> CTTTACCCTACTGGTAAATCCGCGACCTGCTC;> AAACGAGATTGAGTAAACATCGACGGATAGCTATACCGGGGGTTTCTG;> GAACCGCCCCCCCTGCCTCATTTGCCGCCAGCCGGCCAGAGGGTTACC;> GTATAAACGTACCAGGTATAGCCCGGAATAGGGTCACCAGGAATCCCCTGCGGGAT;> CTATTTCGGAACCTATGAGAAGGAGGAGGTTTGGCTGAGATTTTT;> TGATGATAAATGCCGGGAAAGGGGCTCTTCGCTATTACGCCAAGAGAA;> ATGGCTTTTAACGGGGTCAGTGCCATGACCAT;> TAAAGCCAATTCACAACCACCCTCAGAGCCGC;> CACGACGTCGTTTTAAAACGAGGCGCAGACGG;> CGGAAACATCCCGGAATTTGTGAGGGATCCCCATGCGGCGAAAGAAAC;> TGATAGACGGTTTTTCGCCCTTTGACGTTGGAGTCCACGTTCTTTAATAGTGGACTCTTGTTCCAAACTGGAACAACACTCAACCCTATCTCGGGCTATTCTTTTGATTTATAAGGGATTTTGCCGATTTCGGAACCACCATCAAACAGGATTTTCGCCTGCTGGGGCAAACCAGCGTGGACCGCTTGCTGCAACTCTCTCAGGGCCAGGCGGTGAAGGGCAATCAGCTGTTGCCCGTCTCACTGGTGAAAAGAAAAACCACCCTGGCGCCCAATACGCAAACCGCCTCTCCCCGCGCGTTGGCCGATTCATTAATGCAGCTGGCACGACAGGTTTCCCGACTGGAAAGCGGGCAGTGAGCGCAACGCAATTAATGTGAGTTAGCTCACTCATTAGGCACCCCAGGCTTTACACTTTATGCTTCCGGCTCGTATGTTGTGTGGAATTGTGAGCGGATAACAATTTCACACAGGAAACAGCTATGACCATGATTACGAATTCGAGCTCGGTACCCGGGGATCCTCAACTGTGAGGAGGCTCACGGACGCGAAGAACAGGCACGCGTGCTGGCAGAAACCCCCGGTATGACCGTGAAAACGGCCCGCCGCATTCTGGCCGCAGCACCACAGAGTGCACAGGCGCGCAGTGACACTGCGCTGGATCGTCTGATGCAGGGGGCACCGGCACCGCTGGCTGCAGGTAACCCGGCATCTGATGCCGTTAACGATTTGCTGAACACACCAGTGTAAGGGATGTTTATGACGAGCAAAGAAACCTTTACCCATTACCAGCCGCAGGGCAACAGTGACCCGGCTCATACCGCAACCGCGCCCGGCGGATTGAGTGCGAAAGCGCCTGCAATGACCCCGCTGATGCTGGACACCTCCAGCCGTAAGCTGGTTGCGTGGGATGGCACCACCGACGGTGCTGCCGTTGGCATTCTTGCGGTTGCTGCTGACCAGACCAGCACCACGCTGACGTTCTACAAGTCCGGCACGTTCCGTTATGAGGATGTGCTCTGGCCGGAGGCTGCCAGCGACGAGACGAAAAAACGGACCGCGTTTGCCGGAACGGCAATCAGCATCGTTTAACTTTACCCTTCATCACTAAAGGCCGCCTGTGCGGCTTTTTTTACGGGATTTTTTTATGTCGATGTACACAACCGCCCAACTGCTGGCGGCAAATGAGCAGAAATTTAAGTTTGATCCGCTGTTTCTGCGTCTCTTTTTCCGTGAGAGCTATCCCTTCACCACGGAGAAAGTCTATCTCTCACAAATTCCGGGACTGGTAAACATGGCGCTGTACGTTTCGCCGATTGTTTCCGGTGAGGTTATCCGTTCCCGTGGCGGCTCCACCTCTGAAAGCTTGGCACTGGCCGTCGTTTTACAACGTCGTGACTGGGAAAACCCTGGCGTTACCCAACTTAATCGCCTTGCAGCACATCCCCCTTTCGCCAGCTGGCGTAATAGCGAAGAGGCCCGCACCGATCGCCCTTCCCAACAGTTGCGCAGCCTGAATGGCGAATGGCGCTTTGCCTGGTTTCCGGCACCAGAAGCGGTGCCGGAAAGCTGGCTGGAGTGCGATCTTCCTGAGGCCGATACTGTCGTCGTCCCCTCAAACTGGCAGATGCACGGTTACGATGCGCCCATCTACACCAACGTGACCTATCCCATTACGGTCAATCCGCCGTTTGTTCCCACGGAGAATCCGACGGGTTGTTACTCGCTCACATTTAATGTTGATGAAAGCTGGCTACAGGAAGGCCAGACGCGAATTATTTTTGATGGCGTTCCTATTGGTTAAAAAATGAGCTGATTTAACAAAAATTTAATGCGAATTTTAACAAAATATTAACGTTTACAATTTAAATATTTGCTTATACAATCTTCCTGTTTTTGGGGCTTTTCTGATTATCAACCGGGGTACATATGATTGACATGCTAGTTTTACGATTACCGTTCATCGATTCTCTTGTTTGCTCCAGACTCTCAGGCAATGACCTGATAGCCTTTGTAGATCTCTCAAAAATAGCTACCCTCTCCGGCATTAATTTATCAGCTAGAACGGTTGAATATCATATTGATGGTGATTTGACTGTCTCCGGCCTTTCTCACCCTTTTGAATCTTTACCTACACATTACTCAGGCATTGCATTTAAAATATATGAGGGTTCTAAAAATTTTTATCCTTGCGTTGAAATAAAGGCTTCTCCCGCAAAAGTATTACAGGGTCATAATGTTTTTGGTACAACCGATTTAGCTTTATGCTCTGAGGCTTTATTGCTTAATTTTGCTAATTCTTTGCCTTGCCTGTATGATTTATTGGATGTTAATGCTACTACTATTAGTAGAATTGATGCCACCTTTTCAGCTCGCGCCCCAAATGAAAATATAGCTAAACAGGTTATTGACCATTTGCGAAATGTATCTAATGGTCAAACTAAATCTACTCGTTCGCAGAATTGGGAATCAACTGTTATATGGAATGAAACTTCCAGACACCGTACTTTAGTTGCATATTTAAAACATGTTGAGCTACAGCATTATATTCAGCAATTAAGCTCTAAGCCATCCGCAAAAATGACCTCTTATCAAAAGGAGCAATTAAAGGTACTCTCTAATCCTGACCTGTTGGAGTTTGCTTCCGGTCTGGTTCGCTTTGAAGCTCGAATTAAAACGCGATATTTGAAGTCTTTCGGGCTTCCTCTTAATCTTTTTGATGCAATCCGCTTTGCTTCTGACTATAATAGTCAGGGTAAAGACCTGATTTTTGATTTATGGTCATTCTCGTTTTCTGAACTGTTTAAAGCATTTGAGGGGGATTCAATGAATATTTATGACGATTCCGCAGTATTGGACGCTATCCAGTCTAAACATTTTACTATTACCCCCTCTGGCAAAACTTCTTTTGCAAAAGCCTCTCGCTATTTTGGTTTTTATCGTCGTCTGGTAAACGAGGGTTATGATAGTGTTGCTCTTACTATGCCTCGTAATTCCTTTTGGCGTTATGTATCTGCATTAGTTGAATGTGGTATTCCTAAATCTCAACTGATGAATCTTTCTACCTGTAATAATGTTGTTCCGTTAGTTCGTTTTATTAACGTAGATTTTTCTTCCCAACGTCCTGACTGGTATAATGAGCCAGTTCTTAAAATCGCATAAGGTAATTCACAATGATTAAAGTTGAAATTAAACCATCTCAAGCCCAATTTACTACTCGTTCTGGTGTTTCTCGTCAGGGCAAGCCTTATTCACTGAATGAGCAGCTTTGTTACGTTGATTTGGGTAATGAATATCCGGTTCTTGTCAAGATTACTCTTGATGAAGGTCAGCCAGCCTATGCGCCTGGTCTGTACACCGTTCATCTGTCCTCTTTCAAAGTTGGTCAGTTCGGTTCCCTTATGATTGACCGTCTGCGCCTCGTTCCGGCTAAGTAACATGGAGCAGGTCGCGGATTTCGACACAATTTATCAGGCGATGATACAAATCTCCGTTGTACTTTGTTTCGCGCTTGGTATAATCGCTGGGGGTCAAAGATGAGTGTTTTAGTGTATTCTTTTGCCTCTTTCGTTTTAGGTTGGTGCCTTCGTAGTGGCATTACGTATTTTACCCGTTTAATGGAAACTTCCTCATGAAAAAGTCTTTAGTCCTCAAAGCCTCTGTAGCCGTTGCTACCCTCGTTCCGATGCTGTCTTTCGCTGCTGAGGGTGACGATCCCGCAAAAGCGGCCTTTAACTCCCTGCAAGCCTCAGCGACCGAATATATCGGTTATGCGTGGGCGATGGTTGTTGTCATTGTCGGCGCAACTATCGGTATCAAGCTGTTTAAGAAATTCACCTCGAAAGCAAGCTGATAAACCGATACAATTAAAGGCTCCTTTTGGAGCCTTTTTTTTGGAGATTTTCAACGTGAAAAAATTATTATTCGCAATTCCTTTAGTTGTTCCTTTCTATTCTCACTCCGCTGAAACTGTTGAAAGTTGTTTAGCAAAATCCCATACAGAAAATTCATTTACTAACGTCTGGAAAGACGACAAAACTTTAGATCGTTACGCTAACTATGAGGGCTGTCTGTGGAATGCTACAGGCGTTGTAGTTTGTACTGGTGACGAAACTCAGTGTTACGGTACATGGGTTCCTATTGGGCTTGCTATCCCTGAAAATGAGGGTGGTGGCTCTGAGGGTGGCGGTTCTGAGGGTGGCGGTTCTGAGGGTGGCGGTACTAAACCTCCTGAGTACGGTGATACACCTATTCCGGGCTATACTTATATCAACCCTCTCGACGGCACTTATCCGCCTGGTACTGAGCAAAACCCCGCTAATCCTAATCCTTCTCTTGAGGAGTCTCAGCCTCTTAATACTTTCATGTTTCAGAATAATAGGTTCCGAAATAGGCAGGGGGCATTAACTGTTTATACGGGCACTGTTACTCAAGGCACTGACCCCGTTAAAACTTATTACCAGTACACTCCTGTATCATCAAAAGCCATGTATGACGCTTACTGGAACGGTAAATTCAGAGACTGCGCTTTCCATTCTGGCTTTAATGAGGATTTATTTGTTTGTGAATATCAAGGCCAATCGTCTGACCTGCCTCAACCTCCTGTCAATGCTGGCGGCGGCTCTGGTGGTGGTTCTGGTGGCGGCTCTGAGGGTGGTGGCTCTGAGGGTGGCGGTTCTGAGGGTGGCGGCTCTGAGGGAGGCGGTTCCGGTGGTGGCTCTGGTTCCGGTGATTTTGATTATGAAAAGATGGCAAACGCTAATAAGGGGGCTATGACCGAAAATGCCGATGAAAACGCGCTACAGTCTGACGCTAAAGGCAAACTTGATTCTGTCGCTACTGATTACGGTGCTGCTATCGATGGTTTCATTGGTGACGTTTCCGGCCTTGCTAATGGTAATGGTGCTACTGGTGATTTTGCTGGCTCTAATTCCCAAATGGCTCAAGTCGGTGACGGTGATAATTCACCTTTAATGAATAATTTCCGTCAATATTTACCTTCCCTCCCTCAATCGGTTGAATGTCGCCCTTTTGTCTTTGGCGCTGGTAAACCATATGAATTTTCTATTGATTGTGACAAAATAAACTTATTCCGTGGTGTCTTTGCGTTTCTTTTATATGTTGCCACCTTTATGTATGTATTTTCTACGTTTGCTAACATACTGCGTAATAAGGAGTCTTAATCATGCCAGTTCTTTTGGGTATTCCGTTATTATTGCGTTTCCTCGGTTTCCTTCTGGTAACTTTGTTCGGCTATCTGCTTACTTTTCTTAAAAAGGGCTTCGGTAAGATAGCTATTGCTATTTCATTGTTTCTTGCTCTTATTATTGGGCTTAACTCAATTCTTGTGGGTTATCTCTCTGATATTAGCGCTCAATTACCCTCTGACTTTGTTCAGGGTGTTCAGTTAATTCTCCCGTCTAATGCGCTTCCCTGTTTTTATGTTATTCTCTCTGTAAAGGCTGCTATTTTCATTTTTGACGTTAAACAAAAAATCGTTTCTTATTTGGATTGGGATAAATAATATGGCTGTTTATTTTGTAACTGGCAAATTAGGCTCTGGAAAGACGCTCGTTAGCGTTGGTAAGATTCAGGATAAAATTGTAGCTGGGTGCAAAATAGCAACTAATCTTGATTTAAGGCTTCAAAACCTCCCGCAAGTCGGGAGGTTCGCTAAAACGCCTCGCGTTCTTAGAATACCGGATAAGCCTTCTATATCTGATTTGCTTGCTATTGGGCGCGGTAATGATTCCTACGATGAAAATAAAAACGGCTTGCTTGTTCTCGATGAGTGCGGTACTTGGTTTAATACCCGTTCTTGGAATGATAAGGAAAGACAGCCGATTATTGATTGGTTTCTACATGCTCGTAAATTAGGATGGGATATTATTTTTCTTGTTCAGGACTTATCTATTGTTGATAAACAGGCGCGTTCTGCATTAGCTGAACATGTTGTTTATTGTCGTCGTCTGGACAGAATTACTTTACCTTTTGTCGGTACTTTATATTCTCTTATTACTGGCTCGAAAATGCCTCTGCCTAAATTACATGTTGGCGTTGTTAAATATGGCGATTCTCAATTAAGCCCTACTGTTGAGCGTTGGCTTTATACTGGTAAGAATTTGTATAACGCATATGATACTAAACAGGCTTTTTCTAGTAATTATGATTCCGGTGTTTATTCTTATTTAACGCCTTATTTATCACACGGTCGGTATTTCAAACCATTAAATTTAGGTCAGAAGATGAAATTAACTAAAATATATTTGAAAAAGTTTTCTCGCGTTCTTTGTCTTGCGATTGGATTTGCATCAGCATTTACATATAGTTATATAACCCAACCTAAGCCGGAGGTTAAAAAGGTAGTCTCTCAGACCTATGATTTTGATAAATTCACTATTGACTCTTCTCAGCGTCTTAATCTAAGCTATCGCTATGTTTTCAAGGATTCTAAGGGAAAATTAATTAATAGCGACGATTTACAGAAGCAAGGTTATTCACTCACATATATTGATTTATGTACTGTTTCCATTAAAAAAGGTAATTCAAATGAAATTGTTAAATGTAATTAATTTTGTTTTCTTGATGTTTGTTTCATCATCTTCTTTTGCTCAGGTAATTGAAATGAATAATTCGCCTCTGCGCGATTTTGTAACTTGGTATTCAAAGCAATCAGGCGAATCCGTTATTGTTTCTCCCGATGTAAAAGGTACTGTTACTGTATATTCATCTGACGTTAAACCTGAAAATCTACGCAATTTCTTTATTTCTGTTTTACGTGCAAATAATTTTGATATGGTAGGTTCTAACCCTTCCATTATTCAGAAGTATAATCCAAACAATCAGGATTATATTGATGAATTGCCATCATCTGATAATCAGGAATATGATGATAATTCCGCTCCTTCTGGTGGTTTCTTTGTTCCGCAAAATGATAATGTTACTCAAACTTTTAAAATTAATAACGTTCGGGCAAAGGATTTAATACGAGTTGTCGAATTGTTTGTAAAGTCTAATACTTCTAAATCCTCAAATGTATTATCTATTGACGGCTCTAATCTATTAGTTGTTAGTGCTCCTAAAGATATTTTAGATAACCTTCCTCAATTCCTTTCAACTGTTGATTTGCCAACTGACCAGATATTGATTGAGGGTTTGATATTTGAGGTTCAGCAAGGTGATGCTTTAGATTTTTCATTTGCTGCTGGCTCTCAGCGTGGCACTGTTGCAGGCGGTGTTAATACTGACCGCCTCACCTCTGTTTTATCTTCTGCTGGTGGTTCGTTCGGTATTTTTAATGGCGATGTTTTAGGGCTATCAGTTCGCGCATTAAAGACTAATAGCCATTCAAAAATATTGTCTGTGCCACGTATTCTTACGCTTTCAGGTCAGAAGGGTTCTATCTCTGTTGGCCAGAATGTCCCTTTTATTACTGGTCGTGTGACTGGTGAATCTGCCAATGTAAATAATCCATTTCAGACGATTGAGCGTCAAAATGTAGGTATTTCCATGAGCGTTTTTCCTGTTGCAATGGCTGGCGGTAATATTGTTCTGGATATTACCAGCAAGGCCGATAGTTTGAGTTCTTCTACTCAGGCAAGTGATGTTATTACTAATCAAAGAAGTATTGCTACAACGGTTAATTTGCGTGATGGACAGACTCTTTTACTCGGTGGCCTCACTGATTATAAAAACACTTCTCAGGATTCTGGCGTACCGTTCCTGTCTAAAATCCCTTTAATCGGCCTCCTGTTTAGCTCCCGCTCTGATTCTAACGAGGAAAGCACGTTATACGTGCTCGTCAAAGCAACCATAGTACGCGCCCTGTAGCGGCGCATTAAGCGCGGCGGGTGTGGTGGTTACGCGCAGCGTGACCGCTACACTTGCCAGCGCCCTAGCGCCCGCTCCTTTCGCTTTCTTCCCTTCCTTTCTCGCCACGTTCGCCGGCTTTCCCCGTCAAGCTCTAAATCGGGGGCTCCCTTTAGGGTTCCGATTTAGTGCTTTACGGCACCTCGACCCCAAAAAACTTGATTTGGGTGATGGTTCACGTAGTGGGCCATCGCCC;> TTCGCCATTCAGGCTGCCAGCTTTTTTTT;> TCGATGAACGGTAATCAAGCGCCAGGCGATCGCAGTTTGATTCTAGCT;> TTTTTGGAGCAAACTACAAAGCATTGCCTGCTATTTTAAAAGGGTGAGAAAGG;> TTTTCCGGCACCTCGGCCTCAGGAATTTTTTTTTTGATCGCACTCCAGGGTCAGGATTTT;> ACCAGGCAGGATAGGTGCATCTGCTCCTGTAGTTTTAAATGCAATGCC;> ATCAGCTCGTAAAACTTCAGAAAAGTGCGGGCGATGTGCTGCAAGGCG;> TTTTCCGTGGGATTAAATGTGAGCGTTTTTTTTTTAGTAACAACCCGTTTTTGATATTTT;> ACCAATAGGAACGCCATTTTGTTATTTTTTTTTTAAATTCGC;> TTTTCAACTAAAATATAATGCTGTATTTTTTTTTTGCTCAACATGTTTAGAGCTTATTTT;> TCTGGAAGTTTCATTCATAGTAGTGCAAAGAA;> AGCATTAACATCCAATATTTGGGGTTTTTTTTCGCGAGCT;> TAGTTTGATTAGCAAAAATCGGTTGTACCAAACTACAGAGTAAAATGT;> CCATTAGAGCAAGGATAAAAATTTGGTAATAG;> TCAATAACATATTTTCAATACTTTTCCACAGAGAAAGACAGCATCGGA;> CATCAACAACAAACGGCGGATTGACCGTAATGCATATAAC;> CCAGCTTTAGTAGATTAGTTGATTCCCAATTCTAAATATGTTTTT;> TCAAAAATGCAAATGGGAAAAGGTGGCATCAATTCTACTAATTTTTTA;> AAGCAAATCGTTAATAAAAGATTCTGCGGGAGCCAATACTGCGGAATC;> GGGGACGAGTAACCGTCACGTTGGTGTAGATGCGGATTCTTTTTT;> CCACCACCGCAGGTCAGACGATTGTTTGCTCAAGTTAATGCTCAAATG;> CACCAGAAAACCTCACAGCGCAGTCGCAGAAACAGCGGAT;> TTTTTGCCACCCTAACCGCCTCCCTCTTTTTTAGAGCCGCCACCCCCAGAGCCTTTTT;> TTTTTTAGAGAGAACCAGACCGGAATTTTTTTTTTGCAAACTCCAACAGAACGAGTTTTT;> TACCTTTAGGGTAACGCGCAACTGTTGGGAAG;> GATAAATTCAGGAGTGTGTAAAACACGGTGTACAGACCAGATCTTGAC;> AGAGGGTAGTACCCCGGATTGTATATTAAATTTTTGTTAA;> AGGTTGAGAGAGCCGCCGCCAGCATGAGAGATCTTTCAGACGTCATAC;> CACCATCAAAATATCGTGACTATTATTATACCAAGCGCGA;> CCGGAGACAACAGGAAGTTGATAAAGCATGTCAATCATATGAGAGTCTTTTTT;> CGGATAAGTGCCGTCGTTGACAGGCCAGTAAGGGTGGAGC;> TTAGGATTAGCGGGGTGCCTTGATGAATGGAA;> TTTTTCTCCTCAATATTCTGAAACATTTTTTTGAAAGTATTAAGATTGCCATCTTTTT;> TTTTAGAGGTCACGGATTGCATCAATTTTTTTTTTAAAGATTAAGAGGACGGAACATTTT;> TTTTTGCGATTGCTCCGGCGCATCCGACAGTAGCTTCTGGTGCCGGAA;> ATTTCAACTACATTTCAATTCGCGTCTGGCCTGCCCCAAAAGTCAAAT;> AAGCCTTTGACCCTGTAAATCATACAGGCAAG;> TACAAACTATAGTTAGCGTAACGATTGAAAATGCCGCTTTATGACAAC;> TTTTTATAGGAACGCCACCACCCTCATTTTTTTTTTCAGGGATAGGGCATTTTTTTTT;> TTTTATTGCTGAAAAATAGCGAGAGTTTTTTTTTTGCTTTTGCAAAAGGACGACGATTTT;> TTTTCTAAAGGAACAGTTTCAGCGGTTTTTTAGTGAGAATAGAACCTTTAGCTTTTT;> TT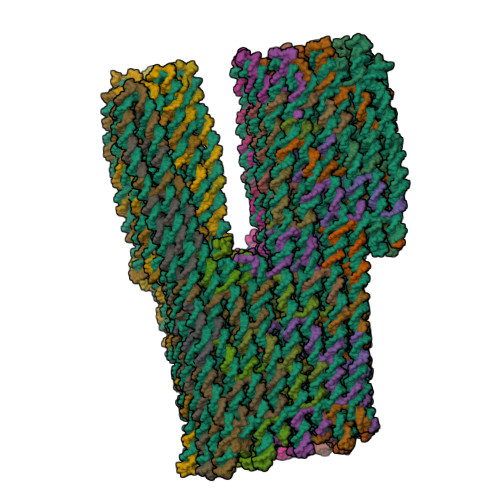TTAGCCTTTATAACCGATATATTTTTTTTTTTTCGGTCGCTGAGGCGTCTGGTCTTTT;> AGCTTGCTTTCGAGGTCGCCGACATGGGATTTTGCCGGACAGAGCACA;> CCCACGCAATTGTATCAAAAGGCTCCAAAAGGTTTTT;> GATAGTTGGAATTTCTTAATAATTTTTTCACGTCTAAAGT;> TGCTAAACAACTTTCAATTGCGAATAAACAGCAGGAACAATTTT;> GCTTTGAGTAAACGGGTAAAATACCGCCAAAACATTCAAC;> TCAGCAGCCAGCCCTCACAACGCCTGTAGCATAGAGGGTT;> TTTCTGTAACCCTCAGGTTAAACGATGCTGATCAGATGCCTTGCCCTGTTACCAGA;> AAATGAATTTTGTCGTCGTAACACTGAGTTTCTGTATCAC;> CCAGAGGGTTAGAACCTAAAGCTAATTAAGCAATAAAGCCGTACGGTG;> AACCGCCACCCTCAGACCATGTACCTTTCCAGCAAGCCCATTTTT;> TTTATTACGCATCAAAAATGAAAATTTTTTTTTTTAGCAGCCTTTACTCTTTCCTTTTTT;> TTTTGGGTGCCTCCATCACCCAAATTTTTTTTTTTCAAGTTTTTTGGGCAAACTATTTTT;> CACATTAATTGCGTTGAAACAGGGTAAGAAACACCAAGTA;> CGCTCACTGCAAACGTAGGGAGGGAAGGTAAA;> GTCGTGCCGAACAAAGCGGCTGGTAATGGGTA;> TTTTACCCAAAACTGAACACCCTGATTTTTTTTTTACAAAGTCAGAGGAATAAGAGTTTT;> TTTTTCGGCCAACGTTCCAGTACTCCAACAATCGTCTGAAATGGAAAACATCG;> AAGTAAGCCAAAAGAATTGCAGCATAACCTCCGGCTTAGGCAAATCCA;> TTTAAGAAAGGAAACCGAGGAAACGCCCGCTT;> AAGCCCTTTCGATAGCAGCACCGTGTAGCGCGCCACGCAATTGATACC;> ATCGGCGAAACGTACACAGAGCCAACAAATAATCAGAACCTTTTT;> ACAGATGAGACGGCCAGTGCCAAGCAGCTGGC;> TGGTGAAGCCAACTTTTTCTTCGCGTCCGTGACACACAACTTTTT;> TTTTTACCACCGGTAGAAAATTCATATTTTTTTGGTTTACCAGCGATTTTGTCTTTT;> TTTTTAGTAAATTAAGGCTTGCCCTGTTTTTTTTTTACGAGAAACACCAACCTTCAT;> CGAACTGATCATCGCCGTCACTGCGCGCCTGTAAAGCCTGTTTTT;> ATCAAAATATTAGCGTAGTACCGCCACCCTCACGTACTCA;> TTTTTTTTTCATATATTGACGGAAATTTTTTTTATTCATTAAAGGGACTCCTTTTTT;> TTTTTACATTATTAAAATCTACGTTATTTTTTTTTTATAAAACGAACTAAATTTCAA;> GATTTGTACCTAAAACCACTGGTGTGTTCAGCTAATGAATTTTTT;> CGCACAGGCGGCCTTTAGTGATGAAATTTCTG;> TCTTTGACGTTTCCATGACTAAAGACTTTTTCTCAGAGCAGATGGCTTTGCGAACG;> TACACTAAAACACTCAGAATACCAGGAATTAC;> GAAAGAGGACTACGAAACGAGGGTAGCAACGGAACATTAT;> GCGGTCCGATAAAAAAGGTGCCCCCTGCATCAGACGATCCATCCCTTA;> TTTTTCGGTCATAAAAATCACCAGTATTTTTTGCACCATTACCATAACGGAATTTTTT;> TTTTTTAAAAACCAACACTATCATAATTTTTTTTTTCCCTCGTTTACCAATCAGTTG;> GTAATGCCCAAAAGAATTAGACTGAATCAGGTTGAGTAATGTGTAGGT;> GGCACCAATTTTTTCGAAGGTTTCTTTGCTCGTCATAAACATACATAA;> TCTCGTCGCTGGCAGCCGTCACCCAGTTAAAGCTCCAAAAGGTTTATC;> CTCCGGCCTTGTAGAAGGTCACTGGCATCAGCTTCACCAGTGAGACGG;> TTTTTGTCAGACTAATCAGTAGCGACTTTTTTAGAATCAAGTTTGGAAATAGCTTTTT;> TTTTAGCAGCAACTTTCGCACTCAATTTTTTTTTTTCCGCCGGGCGCGTTTGCGTATTTT;> GGCAGCACCGTCGGTGGGTGTCCATGAAACCA;> GGGGTCATTGCAGGCGCCGCAAGATGGTGCTGTTGCAGGG;> GTTGCGGTATGAGCCGCGTCAGCGATGCCAACAACCATCG;> GAGGCATAGTAAGAGCATGAGGAAAAAGATTCAAGTTTTGAAGCAAAG;> GTCACCAAAGCCATTTTCCAGTCGGGAAACCTCCGTCTATTAGCCCGA;> TAGCAAGGCCGGAAACTCCTCATAAGGGTAAA;> TAATGCAGTAAGAACTAACAAAGTACAACGGAAAATCAAAGATAGCGT;> AAATCGTTGCGGTGCCATCCCGTAAAAAAAGCCTTTAAACTATTCATT;> AACGGCATTGCCGTTCCGGCAAACGTCATAAAAGTTCAGAGATATAAG;> GGGAATTAGAGCCAGCGCCCCCTTTTTTCATCACGTTAGT;> TGGGAAGAACAGGTAGGATGGTTTAAGCCCGAAAGACTTCATATGATACTCATATA;> GGCTCATTTTACCTTATGCGATTTTTACCCAATCAATCAT;> CCGACTTGACCGATTGAGAAAATACATACATA;> ATTGTGAAATACCAGTCAGGACGTAGATTTAG;> GCACTCTGTCACGGTCCTCACGGATTTCTCCGCGCCACGGGAACGGAT;> CAGTGAATGGGCTTGAGCTGGCTGCCAGGGTTTTCCCAGTATTAAGTTTTCAACCG;> AACAAAGCTGCTCATTCTTTAATCCATGTTACCCCCAGCGATAGTCAG;> ATCAACGTAAGAACCGGATATTCACGTGCCTGGAAAGAGGAAGGGAAC;> CCAGCACGAGCGCAGTTGATAAATTGTGTCGAATAAGTTT;> GGCCGTTTTGGTGCTGAGTTGGGCGGTTGTGTCAGTGCCCTTACCGTT;> GACATTCAGGGTACCGTCCTGTGTGAAATTGTGGAAGGGATCGGAACC;> CCAAAGACAAAAGGGCCAAACTTATTTACCAG;> CAAGAGTAGCGCATAGTTAGCCGGTTCGAGCTTCAAAGCG;> GCCTCCTCACAGTTGAAGATAGACAAAAGAGACTCTGAAT;> AGCTCGAATTCGTAATGCGCCATGCACCGGAAATCCTCAT;> TTTACAATCAATAATTTGCCAGTTTTTTTTTTTTACAAAATAAACAGGCGTCTTTTTTTT;> TTTTTATACGAGCATTTAGAGAAAGCCGGCCGCGCTTAATGCGCC;> GCAAAGACAATCCAAAAGAAAGCGAGCGGTCACGCTGCGC;> GTATGTTAATGATTAATGAATTATCACCGTCA;> TTTTTCCAGAGCCATCCTGAATCTTATTTTTTTTTTCCAACGCTAACGAGCGCCCAA;> TTTTTGTAAAAGATGAGAAGTGTTTTTTTTTTTTTTTATAATCAGTGAGTTTCCTCG;> GTAATAACATCACTTGAAGAACGCAGGTTTTG;> CCTGAGTACACACCCGCGAACGTGGCGAGAAATATCCGCTAACATATA;> CCGTTTTTCCGCACTCGAAAAATAAATAAACAACATGTTCTAATTGAG;> ATTTTCATAAATCAGATATTTTGCACCCAGCTACAATTTTGGGCGCTG;> CGTAGGAAGCAAGTGTAAAGGAGCGGGCGCTACATGGTCAATAAGTTT;> TCATTACCCCATATTATTTATCCCACCACGGATAGCTGTT;> ATCGAGAAATCCAGAATGGCCCACTACGTGAAAATGAGTGTAAAGTGT;> TTTTTTATCATTCTGTAGAAACCAATTTTTTTTTTTCAATAATCGGCTGAAGTAATT;> TCTTACCGTGATTGCCCCAGCTTACGGCTGGAGTGCCATCACGGAACG;> TTTTAATAGCTAGCCCAATAATAAGTTTTTTTTTTAGCAAGAAACAATAATACCGATTTT;> TTTTTTTGGGCGCTTGCCCCAGCAGGCGAATCAAAAT;> GGTTTAACTGTTTGGATTATATTTTTTTTTTCTTCTGAATAATGTCAATATATTTTT;> AGCGGTCCACGCTGGTCAGGGTGGAGAGGCGG;> TGAGAGAGGATAACCCTAAGAATAAACACCGGAACTTTTT;> TGCACGTATAATACATTTGAGGATTAGAGCCG;> AAATCGGCAAAGAAACCACCAGAAATAGCGATGTGAATTTTAGAATCCTTTTT;> AAAATCCCTTATAAATAGATAGCCTTTTTCTT;> TTACAAACTTGAGGAAGGTTATTTTTTTTTTTCTAAAATATCTTCAACAGTTTTTTT;> ATTAGACTAGAACCTACCATATCAATTGCGTA;> ATCAGAGAAAGCGCATACGCTCATGGAAATACAATCGCCA;> TAGACGGGAGAATTAAGAACTGGCGCAATAAT;> TAAAAGGGTAGGAGCACTAACAACTAATAGATTTAGAAGTTTAAATCCTGATTATC;> ATTCACCAGTCACACGAGATAGAACACCGCCTTGAAAAATCTGAGCAA;> CTACATTTTTACTAGAGATAGGGTTGAGTGTTGCGCGGGGAGCTGCAT;> TTTTTAATATAAATTAGGCAGAGGCATTTTTTTTTTTTTTCGAGCCAGTAATTCTTA;> TTTTGAAAGGAAAATCAATATCTGGTTTTTTTTTTTCAGTTGGCAAATCAAATATCTTTT;> TTTGCCCGAGTATTAACCCTTCTGATATTTTTCTAAAGCATCACCTTG;> AACGTTATATTGGCAGTCAATAGACTATTAAAGAACGTGGTTGGAACAAAAGTTTG;> AGTAACATCCAGCAGAAGATAAAACGAACTGATTTTT;> TATCATTTTGACGCTCGTCAAAGGGCGAAAAA;> AAAAGCCTGTTTAGTAAAGCCAACTATTTAAC;> TTTTTCCGTGTGACTTCTGACCTAAATTTTTTTTTTTTTAATGGTTTGATATGTAAA;> TTTTATCCTGATAAATTAATTACATTTTTTTTTTTTTAACAATTTCATAAACATCATTTT;> GTAACAGTACCTTTTATGCTTTGACAGTACATCTGTAAATGAATGGCT;> GAAACAATAAATCCTGAAACAGAAATAAAGAAAAATTATTCATATTCC;> CATAGGTCAGTCAATAAGCTTAGATTAAGACGACGAACCA;> TCGCGCAGGTCAGATGAATATACAGATTTTCA;> ATCGCAAGACAAAGAACTGAGAAGTGAGAGACTGCGGAAC;> TGCTGATGTTGGGTTAGCGTTAAAACAAGAATTGAGTTAA;> CCTTTTTTAGATGATGGCAATTCAGAAGGGTT;> AATGGAAAATACCAAGTCAATTACCGTCGCTATTAATTAA;> CAAATATATTTTAGTTCCAGTATATCATATGCCAGGAAAA;> AATTTCATTAAATAAGTATAACTACTTCACCGCCTGGCCCGCAACAGC;> GCTCAACAGTAGGGCTCGCGAGAAAATCATAATACCTTTT;> GCGTAAGATTATTTACTAATTTTAAGAGTCCATTTGATGGTGGTTCCG;> CCATTAAAAATACCGAAGCTAATGCTGGTAATGAAGAACT;> AACGCCAACTGTCCAGCATTGCAAGGTATTAAGATTTTTTGTTTAACG;> CATGTAATGTACCGACGTTATACAGTAATTGAGCGCTAAT;> CTGAACCTACATTCTGGCCAACAGACCAGTAAAACTCGTA;> TTTTTTAGCCCTAATACGTGGCACAGACAACCTGAAA;> TTTTTAAACCCTCGAGAGCCAGCAGCAAAGCAACAGT;> ATTAGTCTTTAATGCGCAGAGGTGATATGTGAGGAGCGGA;> AAGAAGATGATGAAACTTGAATTAGCCACGCTAATTCGAC;> TTTTTTTGAAAACGTGAATAACCTTGCTTAAATCAATAGGCGGTC;> TTTTTAGAAAACAAGGCGAATTATTCATTTTACAAAA;> TTTTCCCTAACGGATTCGCCTGATCATCGGGAATTATCAT;> GTCGAGGTGCCGTAAAAAGGTGGCAGCTAACTTGCAGCCA;> GCACTAAACAGGGCGACAATATTACCGCCAGC;> CTAAAGGGAGCCCCCGCGGAAGCACACAATTC;> TATGGTTGCTTTGACGAGAGCGGGGACAGGAA;> TTTTTCGGCCTTGCAGAACGCCAACAATAGATAAGTCGGTATTCT;> ACGACGACATATCCCATCCTAATTTAGCAAGC;> TACGAGCACAAGAACGAAAAGGTAAGAGAGAATAACATAA;> CGGTACGCCAGAATCCGTCTGTCCTAACGTGCGCCACCGATTTTT;> TTAGAATCAGCACGTAATCACGCAAATTAACCGTTGTAGCGGATTTTA;> AGCTAAACAGGAGGCCCCTCCCGAGCTACAGGTTTGATTA;> CTTGCGGGGAGGCGTTTTAGCGAAGATTAAAGAATACTTCGCGCGTAC;> AAGCCTTAAATCAAGAGTAACCACCAAGCAAG;> TTAGTTGCTATAGAAGGCTTATCCCTGAACAA(2S)-2-azanyl-3-(6-methyl-1H-indol-3-yl)propanoic 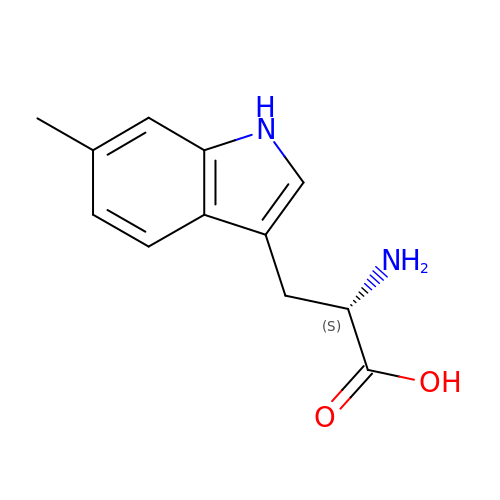acid | C12 H14 N2 O2 | GDMRVYIFGPMUCG-JTQLQIEISA-N>[2x]MKLLLFGYGNVGKAFRKLLHEKRSPELNDVIIGGIVTRRGIMLQDKEDFTPDLEGDVFKAFEKIKPDIIVDVS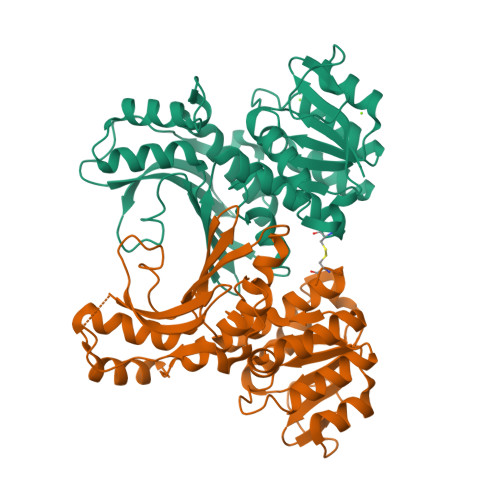SANYNNGEPSLSLYKEAIKDGVNIITTNKAPLALAFNEIFSLARSKGVKIGFQGTVMSGTPSINLYRVLPGSRVIKIRGILNGTTNFILTLMNKGVSFEEALKEAQRRGYAEEDPTLDINGFDAAAKITILANFMIGNSVTIKDVKFEGINRDLPKNEKIKLIAYADEKEVWVKPLPISQDDPLYNVDGVENALEITTDIQSILIRGPGAGPVNAAYGALSDLILLKRDCL>[4x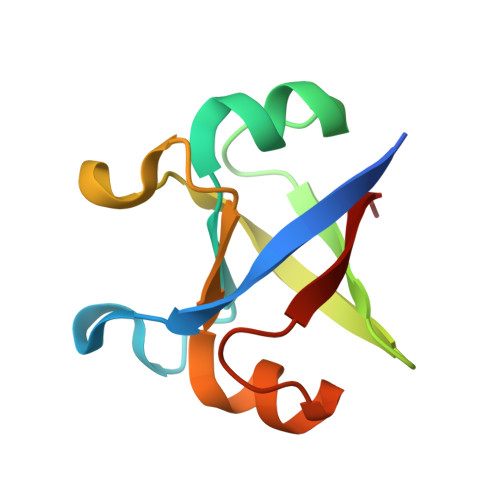]GPMPGKSVVARVAPAHPEDVGKGIVRMDKYERQNLGVSVGDYVEVKKAKSVVARVAPAHPEDVGKGIVRMDKYERQNLGVSVGDYVEVKKA3,5-dideoxy-5-(propanoylamino)-D-glycero-alpha-D-galacto-non-2-ulopyranosonic 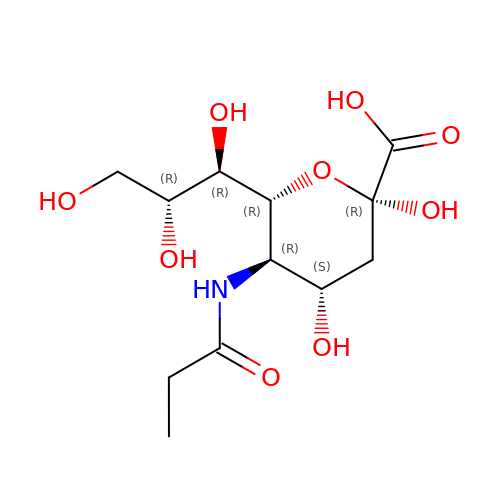acid | C12 H21 N O9 | QZBCMZXFDLYCRV-BLMTXZDNSA-N>MFNSVLDTIGNTPLIRLSKASELTGCDIYGKAEFLNPGQSVKDRAALYIIRDAEKRGLLRPGGVIVEGTAGNTGIGLTMVAKALGYRTAIVIPETQSQEKKDALRLLGAELIEVPAAPYRNPNNYVRLSGRLAEQLAKTEPNGAIWANQFDNTVNRQAHIETTAQEIWRDTSDQIDGFVAAVGSGGTLAGTAIGLKERNHNIKIALADPHGAALHAFYTTGELKAEGDSITEGIGQGRITANLEGFTPDFSYQIPDAEALDILFALVEEEGLCLGGSSGINIAGAIRLAKDLGPGH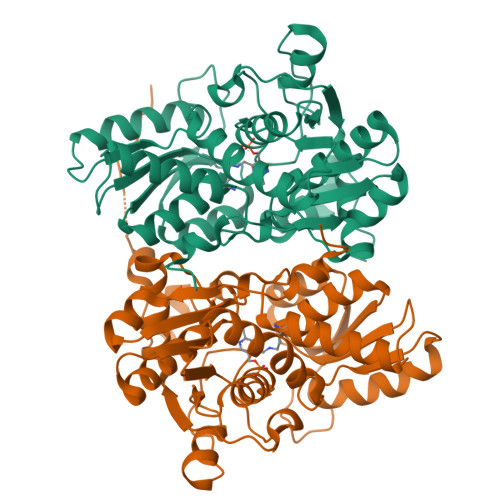TIVTVLCDYGNRYQSKLFNPAFLRGKSLPVPRWLEKKTEIDIPFEGLEHHHHHH[4x]The three largest gene segments of the Thogotoviruses, THOV, DHOV and JOSV are homologous to those of IAV and code for the heterotrimeric polymerase. In this paper we present the atomic structures of the putative PB2 cap binding and 627 domains of THOV and the putative PA N-terminal endonuclease domains of THOV and DHOV. Despite very low sequence homologies, all domains have similar folds to those of the corresponding IAV polymerase domains. However, the critical active site residues in the putative cap binding and endonuclease domains are not conserved in THOV and DHOV and, contrary to the case of IAV polymerase, neither domain shows the expected in vitro biochemical activity.

The corresponding construct (residues 1 to 169) was cloned, expressed, purified and crystallized. THOV PA-Nter comprises four principle β-strands surrounded by six α-helices. Comparison of the two independent molecules in the asymmetric unit of crystal form 1 shows that the region 72–89, including helix α3 and the following loop, is in two very distinct orientations. Interestingly, this asymmetry is also observed in crystal form 2 of THOV PA-Nter in which there are six molecules in the asymmetric unit. These are arranged as three asymmetric dimers, each similar to that observed in form 1, but for the chain in which the 72–89 element is dissociated from the body of the protein, the electron density for the element is lacking, presumably due to mobility. Interestingly, the significant difference in thermal stability behaviour of the THOV and DHOV domains correlates with the enhanced plasticity and much poorer diffracting crystals of THOV PA-Nter. For THOV and DHOV PA-Nter the putative active site is more like an extended groove and furthermore, is positively charged. Our structural and biochemical results therefore strongly suggest that THOV and DHOV PA-Nter domains neither bind divalent cations nor are active endonucleases.

>[6x]GMGSGMAMTDRPDHIDSRVWELSETQEDWITQVHGHVRRVVECWKYTICCLISNMHTHRGAPQYDVFKWQDRSTIEWICSKKKVQYPERDTPDLYDNERAVAYKVLLVSDLSDHSPTSGIYHDLAFNLEGEAEESCALVLRGSQLQDIKGFLCRALEWVVSNNLTQEVVETISGEAK> MSVHALRELFKHKGEKNYEVFSMEDFIGRLESEIGLNDSVVSQGRSLISSISHENFGTVQATDIQDAAAIYNKMQMLVNDYGFERVSSSDPQVRAREERVRENQITAATMAAIACADETKYIRALRGITKAKASNEDHVKVVQHQFNGPAGGIQVFENGVGLENYNEKSQRDFRVVTIGYNLAASRQDEFAERIYPTTVINPIEGGVVQVLPYIAVMKDVYHEVSGVKMDNEEVNMVEAYRDPSILDDESIALIPALDPAGSNADFFVDPALVPPYTIKNEQNLTITTAPLKANVRLDLMGNSNANLLIQRGMLEVSDTIDPAGRLKNLFVLLGGKVVKFKVDRLPRAVFQPDLVGDTRNAVIRFDSDDLVVSGDTTFIDGSADGVINDLKTAKLSLRLSVGFGGTISLSKGDSKFGATDTYVDKVLNEDGQVMDNADPAVKAILDQLTDLAV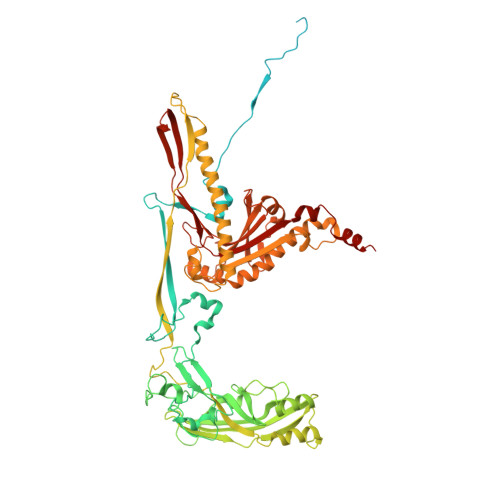IGFELDTRFTNTNRRQRGHLLQTRALQFRHPIPMHAPVTLPMDTMTDEGPGEVVKALTVNTNIRNSNNAVKRMLNYLAQLREVVHNGYNRPKFGIIEGALSAVMRPTYRYKELDLEKVIDTIKSKDRWDDVCAAILNCVKAELFPAHRDSNIEAAFRVISGNQDETPMYLFCSDKEIANYLMTKGDDRTLGAYLKYDIVSTNNQLFDGKLVVIPTRAVQQENDILSWGQFFYVSTVIADLPITRGGHQVTREIAAIPFNLHVNNIPFALEFKITGFQKVMGETQFNGKLADLKP> MSTPPLAASGMAPGPFAGPQAQQAAREVNTASLCRIGQETVQDIVYRTMEIFQLLRNMQLPNGVTYHTGTYQDRLTKLQDNLRQLSVLFRKLRLVYDKCNENCGGMDPIPVEQLIPYVEEDGSKND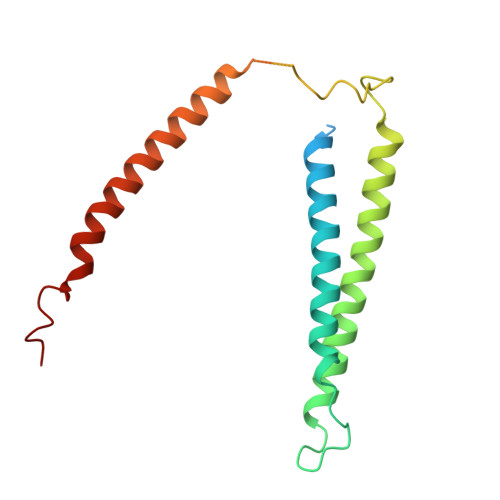DRAGPPRFASEERREIAEVNKKLKQKNQQLKQIMDQLRNLIWDINAMLAMRN>MGHHHHHHSHMKSKFEASIDNLKEIEMNAYAYELIREI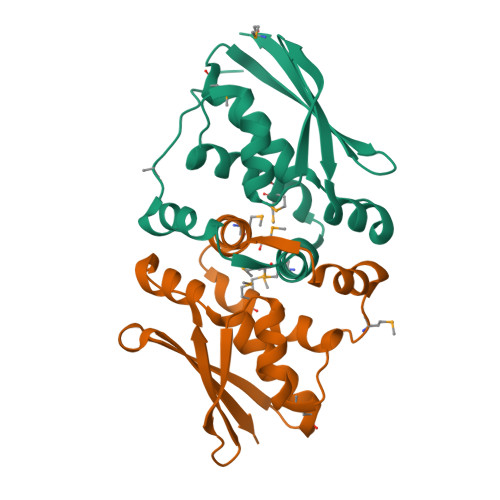VLPDMLGQDYSSMMYWAGKHLARKFPLESWEEFPAFFEEAGWGTLTNVSAKKQELEFELEGPIISNRLKHQKEPCFQLEAGFIAEQIQLMNDQIAESYEQVKKRADKVVLTVKWDMKDPV[2x]> KANRQREPGLGFSFEFTEQQKEFQATARKFAREEIIPVAAEYDKTGEYPVPLIRRAWELGLMNTHIPENCGGLGLGTFDACLISEELAYGCTGVQTAIEGNSLGQMPIIIAGNDQQKKKYLGRMTEEPLMCAYCVTEPGAGSDVAGIKTKAEKKGDEYIINGQKMWITNGGKANWYFLLARSDPDPKAPANKAFTGFIVEADTPGIQIGRKELNMGQRCS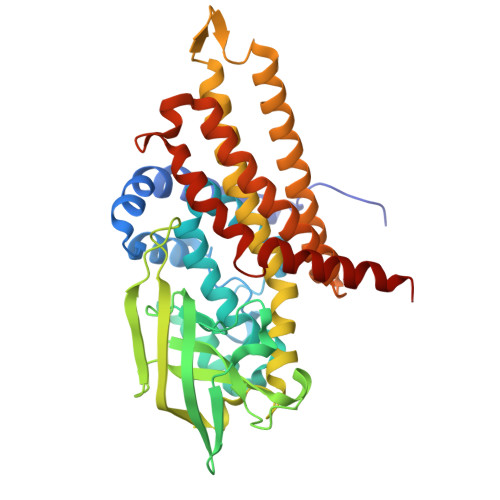DTRGIVFEDVKVPKENVLIGDGAGFKVAMGAFDKTRPVVAAGAVGLAQRALDEATKYALERKTFGKLLVEHQAISFMLAEMAMKVELARMSYQRAAWEVDSGRRNTYYASIAKAFAGDIANQLATDAVQILGGNGFNTEYPVEKLMRDAKIYQIYEGTSQIQRLIVAREHIDKYKN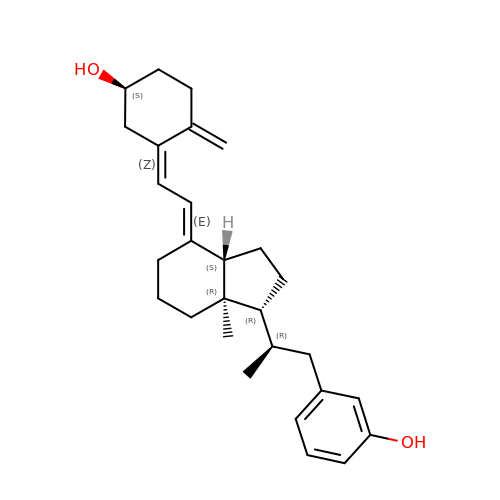3-(2-{4-[2-(5-HYDROXY-2-METHYLENE-CYCLOHEXYLIDENE)-ETHYLIDENE]-7A-METHYL-OCTAHYDRO-INDEN-1-YL}-PROPYL)-PHENOL | C28 H38 O2 | FUULLJKQLABNSA-YPMWTJJSSA-N> MKKNHHHHHHLVPRGSKLASSIVCDSTIENPCIVQDSKTQFSPVIRYREVASIADVYGGNITGINKFHLSGSEQPSEKGWEAIAESISRKMGAETKKVIVLDLRQESHGYLNGRAITLVSVYNWINLGKSNSQSTLDQENWLTGLRSRKIVNGVLTVPQYVAKQYSQGKSMVVSTVKNEEYYVYKKGFDYYRIFISDHRAPLDSEVDALV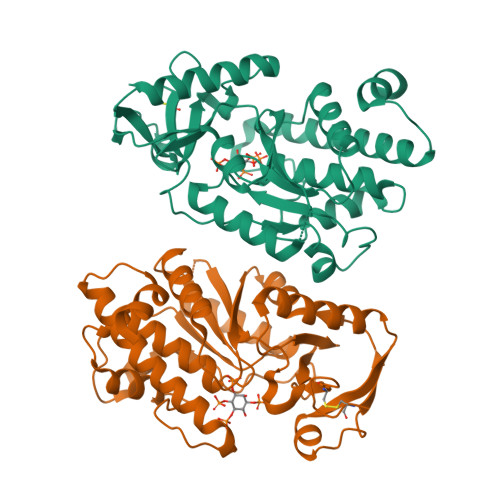ALIKNNPEDTWYHVHSRGGKGRTTTVFAMFDMLKNADKVSFEEIIARQASIPPFYNLMVTNREIPELTPYYEQRLQFLIHFYEFARQSLMGYSGTWSEWKKLNI>MSDSSPTINFINFNQTGTCISLGTSKGFKIFNCEPFGKFYSEDSGGYAIVEMLFSTSLLALVGIGDQPALSAARLRIINTKKHSIICEVTFPTSILSVKMNKSRLVVLLQEQIYIYDINTMRLLHTIETNPNPRGLMAMSPSVANSYLVYPSPPKVINSEIKAHATTNNITLSVGGNTETSFKRDQQDAGHSDISDLDQYSSFTKRDDADPTSSNGGNSSIIKNGDVIVFNLETLQPTMVIEAHKGEIAAMAISFDGTLMATASDKGTIIRVFDIETGDKIYQFRRGTYATRIYSISFSEDSQYLAVTGSSKTVHIFKLGHSMSNNKLDSDDSNMEEAAADDSSLDTTSIDALSDEENPTRLAREPYVDASRKTMGRMIRYSSQKLSRRAA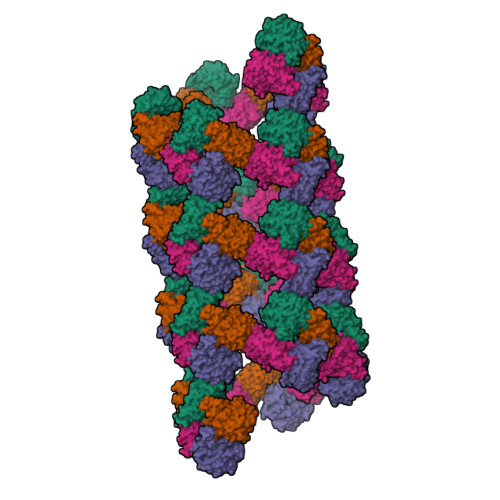RTLGQIFPIKVTSLLESSRHFASLKLPVETNSHVMTISSIGSPIDIDTSEYPELFETGNSASTESYHEPVMKMVPIRVVSSDGYLYNFVMDPERGGDCLILSQYSILMD[4x]> MSAYQNEIKAVAALKEKNGSSWSAINPEYAARMRIQNRFKTGLDIAKYTAAIMRKDMAEYDADSSVYTQSLGCWHGFIGQQKLISIKKHLKTTNKRYLYLSGWMVAALRSDFGPLPDQSMHEKTAVSGLIEELYTFLRQADARELDLLFTGLDAARAAGDKAKEAELLAQIDNFETHVVPIIADIDAGFGNAEATYLLAKKMIEAGACCIQIENQVSDEKQCGHQDG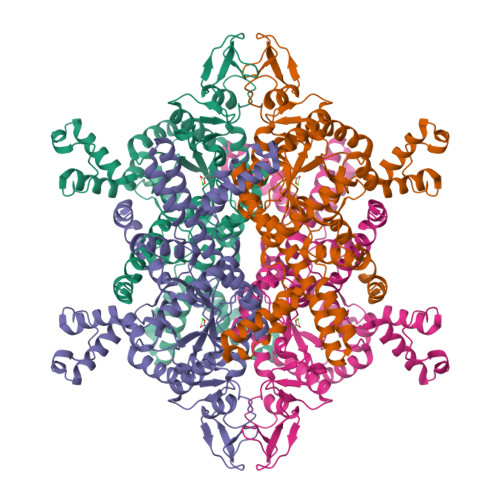KVTVPHIDFLAKINAVRYAFLELGVDDGVIVARTDSLGAGLTKQIAVTNEPGDLGDLYNSFLDCEEISESELGNGDVVIKREGKLLRPKRLASNLFQFRKGTGEDRCVLDCITSLQNGADLLWIETEKPHVGQIKAMVDRIREVIPNAKLVYNNSPSFNWTLNFRQQVFDAFVAEGKDVSAYDRNKLMSVEYDDTELAKVADEKIRTFQRDGSAHAGIFHHLITLPTYHTAALSTDNLAKGYFADEGMLAYVKGVQRQE> MEEPEEPADSGQSLVPVYIYSPEYVSMCDSLAKI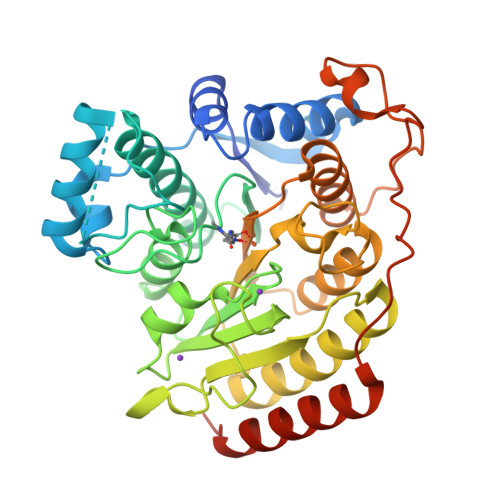PKRASMVHSLIEAYALHKQMRIVKPKVASMEEMATFHTDAYLQHLQKVSQEGDDDHPDSIEYGLGYLCPATEGIFDYAAAIGGATITAAQCLIDGMCKVAINWSGGWHHAKKDEASGFCYLNDAVLGILRLRRKFERILYVDLDLHHGDGVEDAFSFTSKVMTVSLHKFSPGFFPGTGDVSDVGLGKGRYYSVNVPIQDGIQDEKYYQICESVLKEVYQAFNPKAVVLQLGADTIAGDPMCSFNMTPVGIGKCLKYILQWQLATLILGGGGYNLANTARCWTYLTGVILGKTLSSEIPDHEFFTAYGPDYVLEITPSCRPDRNEPHRIQQILNYIKGNLKHVVIEGRGSHHHHHH>[2x]AQCEATIESNDAMQYDLKEMVVDKSCKQ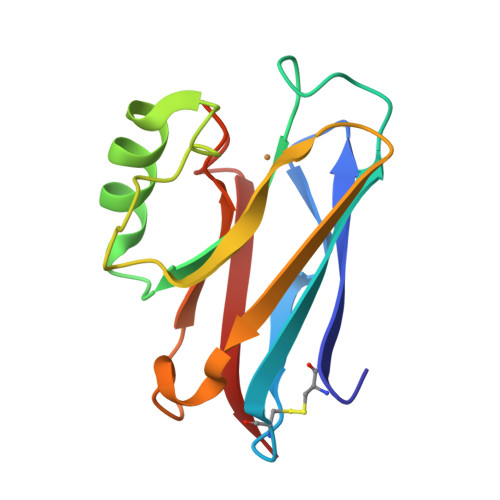FTVHLKHVGKMAKSAMGHNWVLTKEADKEGVATDGMNAGLAQDYVKAGDTRVIAHTKVIGGGESDSVTFDVSKLTPGEAYAYFCSFPGHWAMHKGTLKLSN[[(2R,3S,4R,5R)-5-(6-aminopurin-9-yl)-3,4-bis(oxidanyl)oxolan-2-yl]methoxy-oxidanyl-phosphoryl] 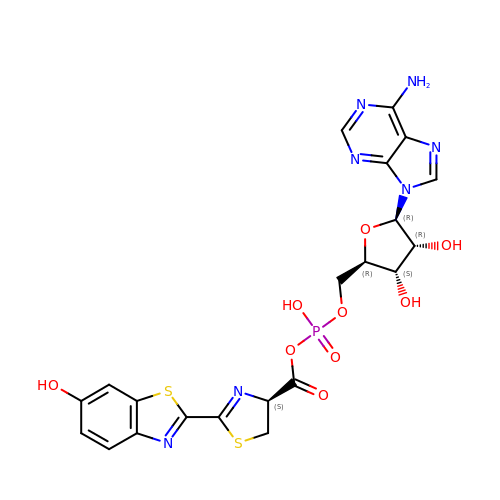(4S)-2-(6-oxidanyl-1,3-benzothiazol-2-yl)-4,5-dihydro-1,3-thiazole-4-carboxylate | C21 H20 N7 O9 P S2 | DVLIEEOCYVGZDS-RIWZETFMSA-N[3-bromanyl-5-(carbamimidoylsulfanylmethyl)phenyl]methyl carbamimidothioate | C10 H13 Br N4 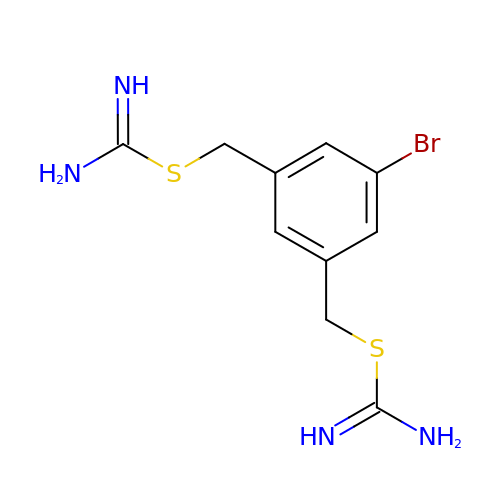S2 | KHMFYTPEFLUGGV-UHFFFAOYSA-N> ACGGACAG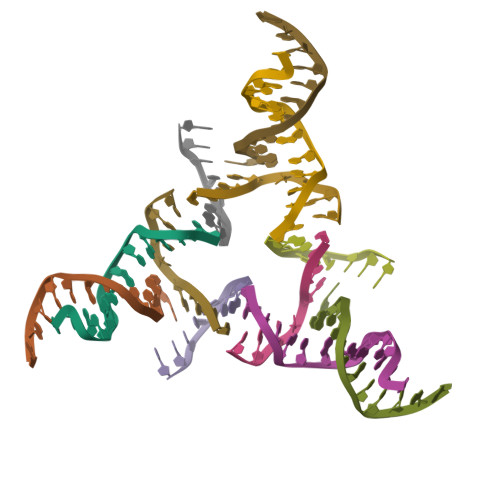AGTGCA;> CACACCGT;> AGTGCACTCTGTG;> TCCTGTG> VTS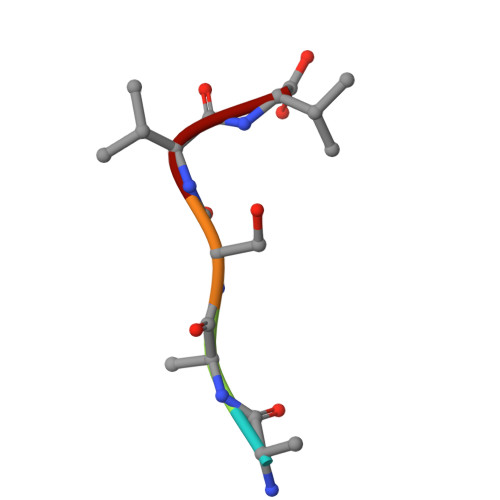VV> MKDEVALLAAVTLLGVLLQAYFSLQVISARRAFRVSPPLTTGPPEFERVYRAQVNCSEYFPLFLATLWVAGIFFHEGAAALCGLVYLFARLRYFQGYARSAQLRLAPLYASARALWLLVALAALGLLAHFLPAALRAALLGRLRTLLPWAHHHHHH

LTC4S catalyzes the conjugation of glutathione (GSH) and leukotriene A4 (LTA4), which is an unsaturated fatty acid that is involved in eicosanoid biosynthesis. There are several defined DDM molecules per 17 kDa monomer of LTC4S and the biologically functional unit of LTC4S is a homotrimer. Dodecyl-β-d-selenomaltoside (SeDDM) is a seleno-detergent with a β-glycosidic seleno-ether in place of the ether moiety in dodecyl-β-d-maltoside. Crystals of a nuclear membrane-embedded enzyme, leukotriene C4 synthase (LTC4S), in complex with SeDDM were prepared and a multiwavelength anomalous diffraction (MAD) experiment was performed.

The SeDDM in the LTC4S crystal exhibited sufficient anomalous diffraction for determination of the structure using MAD phasing. There were three selenium sites: two were found using SOLVE in PHENIX, while the other was manually picked from the anomalous difference Fourier map. Site 1 was between helices IV and V and helices IV* and V* in a twofold symmetry-related molecule. Site 2 was along the transmembrane helices I and III, and site 3 was in the active site of LTC4S. The alkyl chains of the SeDDM molecules were surrounded by hydrophobic residues in all three sites, indicating that hydrophobic interactions are involved in the binding of SeDDM. The SeDDM molecules bound three sites in competition with DDM molecules; therefore, it is possible that the DDM-binding sites were not fully substituted by SeDDM. Site 3 is the putative LTA4-binding site in the active site of LTC4S. The alkyl chain was inserted into the valley between helices composed of hydrophobic residues, including Leu105, Leu108, Tyr109, Ala112, Leu115 and Trp116 of helix IV, Tyr59 of helix II and Val16, Ala20, Leu24 and Ile27 of helix I* in the adjacent monomer. The electron density of maltoside was located next to the thiol group of the GSH. The position of the SeDDM alkyl chain in the putative LTA4-binding site was clearly defined.> MQHNLIAFLSDVGSADEAHALCKGVMYGVAPAATIVDITHDVAPFDVREGALFLADVPHSFPAHTVICAYVYPETGTATHTIAVRNEKGQLLVGPNNGLLSFALDASPAVECHEVLSPDVMNQPVTPTWYGKDIVAACAAHLAAGTDLAAVGPRIDPKQIVRLPYASASEVEGGIRGEVVRIDRAFGNVWTNIPTHLIGSMLQDGERLEVKIEALSDTVLELPFCKTFGEVDEGQPLLYLNSRGRLALGLNQSN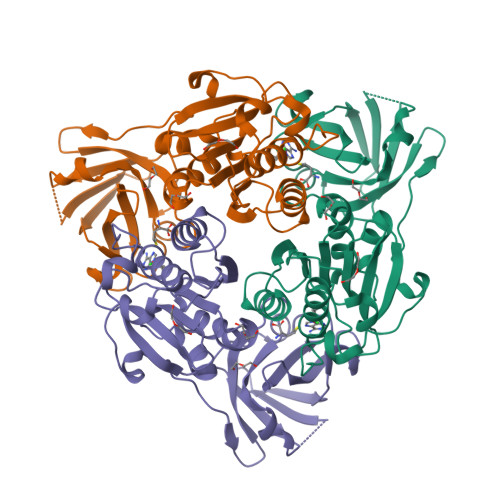FIEKWPVVPGDSITVSPRVPDSNLGPVLG> GSMKSTFKSEYPFEKRKAESERIADRFKNRIPVICEKAEKSDIPEIDKRKYLVPADLTVGQFVYVIRKRIMLPPEKAIFIFVNDTLPPTAALMSAIYQEHKDKDGFLYVTYSGE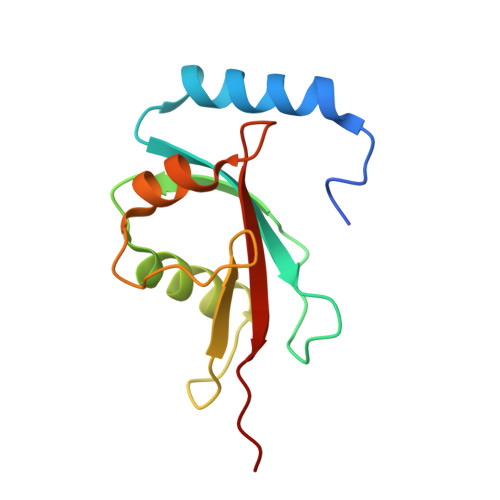NTFG> MERLSEDDPAAQALEYRH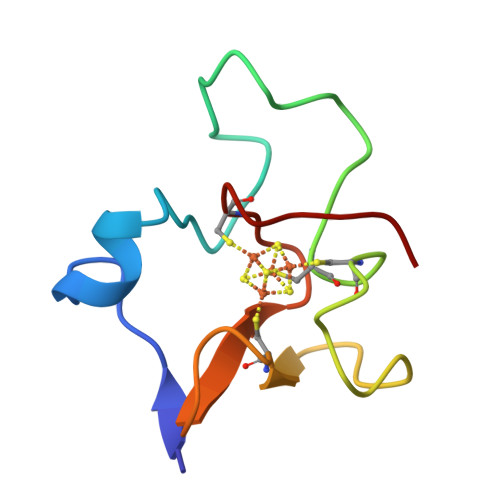DASSVQHPAYEEGQTCLNCLLYTDASAQDWGPCSVFPGKLVSANGWCTAWVAR>[2x]MNTKYNKEFLLYLAGFVDGDGSIIAQIAPNQSYKFKHQLSLTFVVTQKTQRRWFLDKLVDEIGVGYVRDRGSVSDYILS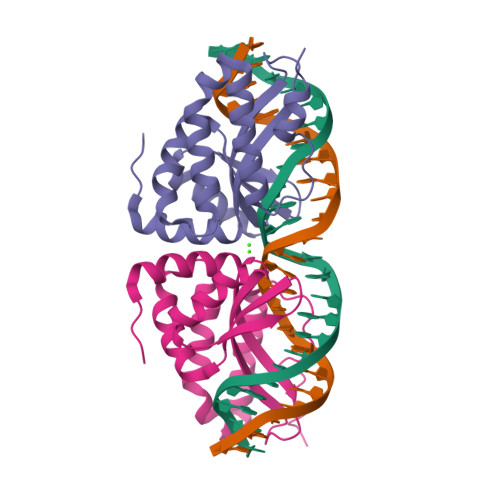EIKPLHNFLTQLQPFLKLKQKQANLVLKIIEQLPSAKESPDKFLEVCTWVDQIAALNDSKTRKTTSETVRAVLD> MACGALLFKGKIPFVVELEGDVNGEVFSVRGNGWGDGSTGKLEIKFVCTTGEVPLAWESLICSMAYGALVFCKYPSNINDFFKSTMPRGYIQERKISYENDGTFD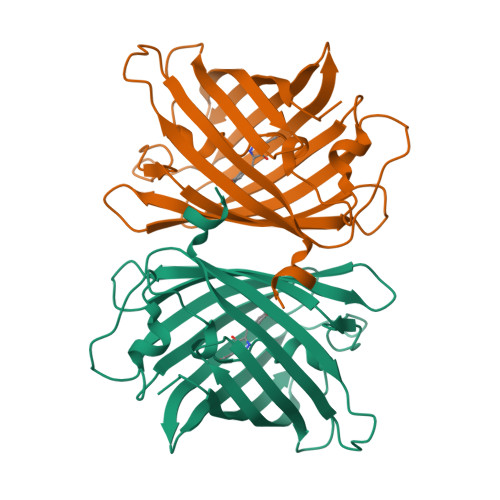VRQEVTYENGALYNRVKFNGSGFRKDGNVLGKKLDLTSIGTCIYIMGNDEGTGLKGVFNKAFKVIGGNRQIASHVQTQTPIGDGLVSIPDYHVMHNHIACSKDPSETRDHIIVKESLRAVDCNTEYM>MSLRITRIRLYKTDLPYVDGSYGWGAGNAITVARASVVVIDTDAGLQGCGEFTPCGENYMIAHSEGVDAFARLAAPQLLGQDPRQVARMERLMDHLVQGHGYAKAPFDAAFWDILGQATGQPVWMLLGGKLCDGAPMYRVAPQRSEAETRAELARHRAAGYRQFQIKVGADWQSDIDRIRACLPLLEPGEKAMADANQGWRVDNAIRLARATRDLDYILEQPCRSYEECQQVRRVADQPMKLDECVTGLHMAQRIVADRGAEICCLKISNLGGLSKARRTRDFLIDNRMPVVAEDSWGGEIASAAVAHFAASTPEE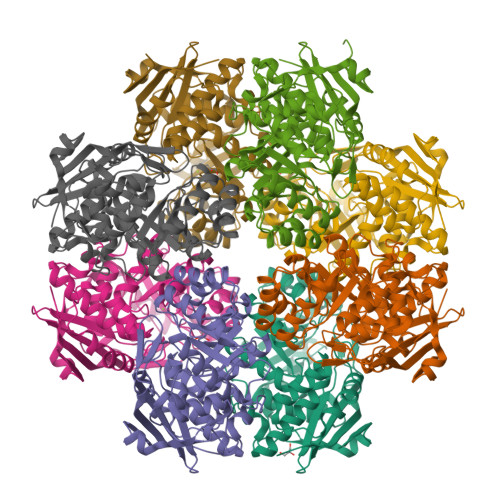FLINSTDLMNYNTRSTGLGGPTVHQGRLYASDTPGLGVTPDFNSLGAPVADWALPEGHHHHHH[8x]>[6x]MSQWSLSQLLSSLHEDIQQRLSVVRKTFGHPGTKGDASENVWID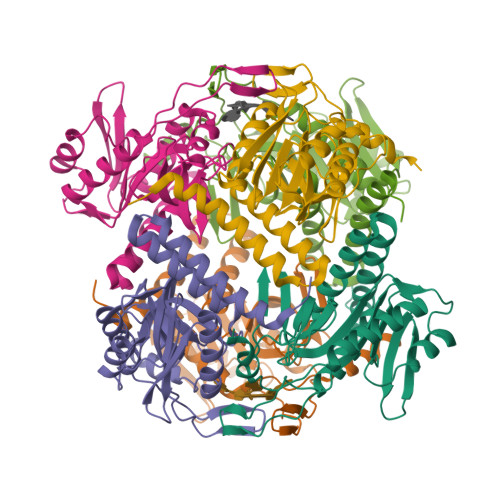MLDTYLPKRYQAAKAHVVDSLGNFSQQINVVVFDRQYSPFIFTYENETIIPAESVYAVFEAKQTADAGLVAYAQEKVASVRRLHRTSLPIPHAGGTYPAKPLIPILGGLLTFESEWSPALGPSMDKALNANLTEGRLDIGCVAAHGHFFYDQASGAYSYTNENKPATAFLFKLIAQLQFSGTVPMIDVEAYGQWLTK> MSATLKDYLNKRVVIIKVDGECLIASLNGFDKNTNLFITNVFNRISKEFICKAQLLRGSEIALVGLIDAENDDSLAPIDEKKVPMLKDTKNKIENE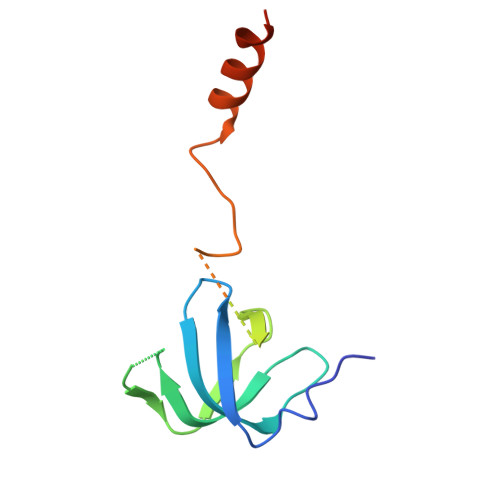HVIWEKVYESKTKHHHHHH> INGNNYVYIDPTQLPYDHKWEFPRNRLSFGKTLGAGAFGKVVEATAYGLIKSDAAMTVAVKMLKPSAHLTEREALMSELKVLSYLGNHMNIVNLLGACTIGGPTLVITEYCCYGDLLNFLRRKRDSFICSKTSPAIMEDDELALDLEDLLSFSYQVAKGMAFLASKNCIHRDLAARNILLTHGRITKICDFGLARDIKNDSNYVVKGNARLPVKWMAPESIFNCVYTFESDVWSYGIFLWELFSLGSSPYPGMPVDSKFYKMIKEGFRMLSPEHAPAEMYDIMKTCWDADPLKRPTF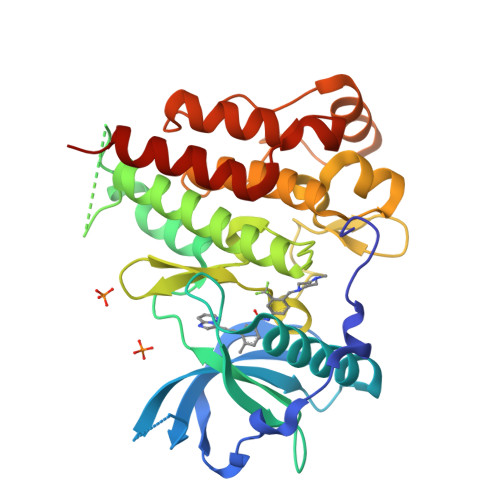KQIVQLIEKQISESTNHI> MNDKEKIDKFIHSNLNDDFGLSVDDLVGKVKGIGRFSAWCGNSSTKIKQVLNAVKSIGVSPALFAAYEKNEGYNGSWGWLNHTSPQGNYLTDAQFVARKLVSQSRQAGTPSWIDAGNPVDFVPASVKRKGNYDFSHNMKNGKVGRAYIPLTAAATWAAYYPEGLQASYNRVQNYGNPFLDAANTILGWGGKIDGKGGSSSGSSSSSSGTSGGLDVVARAFEEFLKKLQDSMQWDLHSIGTDKFFSNQMFTITKTYNNTYRLNMNQKLLDEMKDLISRIDGGSGNDTGADDSDGDHGGKAGKSVAPNGKSGRKIGGNWTYSNLPQKYKDAIEVPKFDPKYLAGSPFVNTGDTGQCTELTWAYMHQIWGKRQPAWDNQVTNGQRVWVVYRNQGARVTHRPTVGYGFSSKPNYLQAMLPGVGHTGVVVAVFKDGSFLTANYNVPPYWAPSRVVEYALIDGVPENAGDNIMFFSGIK;>[3x]VTNEKGQAYTEMLQLFNLLQQWNDFYTAENANNLLVACQQLLINYNEPVIKFINDENEDKSLLQYLAGDDGLAQWQFYKGFYNNYNVHIF

Staphylococcal picoviruses are a group of strictly lytic, short-tailed bacteriophages with compact genomes that are attractive candidates for therapeutic use. Here, we report the structure of the complete virion of S. epidermidis–infecting phage Andhra, determined using high-resolution cryo–electron microscopy, allowing atomic modeling of 11 capsid and tail proteins. The overall structure of the Andhra virion follows that of other phages in this group, with an isometric head (capsid) around 500 Å in diameter (vertex to vertex), connected to a 400-Å-long, straight tail surrounded by 12 appendages. The head has icosahedral symmetry, with the tail attached to a portal structure located at 1 of the 12 fivefold vertices.

To resolve the tip density, we carried out another masked reconstruction focused on the tail tip without the application of symmetry, reaching a resolution of 4.9 Å. This reconstruction revealed a twofold symmetric structure consisting mostly of α helices, with a four-helix bundle inserting into the knob. An AlphaFold model for Andhra gp10 revealed the two expected domains (GyH and CHAP), separated by a helix-sheet-helix linker domain (residues 211 to 277). The three domains were individually fitted into the tail tip reconstruction, revealing a gp10 dimer with the N-terminal GyH domains at the bottom of the tip and the C-terminal CHAP domains at the top. The two α helices of the linker domain fit into the connecting densities between the tip and the knob, with the β sheet penetrating into the gp12 knob protein above. After fitting the gp10 dimer into the tip density, it was clear that the tip contained at least one other, primarily α-helical protein. After subtracting the gp10 density, the remaining density appeared as a flat disc with quasi-threefold symmetry. Closer analysis revealed that the disc was made of three dimers, with the twofold symmetry axis of the tip passing through one dimer and the other two dimers on opposite sides of the tip. We generated AlphaFold models for each of these proteins. gp2, gp4, and gp5 were a poor match for the tail tip density, but gp1 had a compact, α-helical structure that could be fitted as three dimers into the tail tip disc density. The tail tip lysins insert into the knob and stabilize the internal loops that hold back the terminal protein and the DNA, thus coupling cell wall penetration to DNA release.>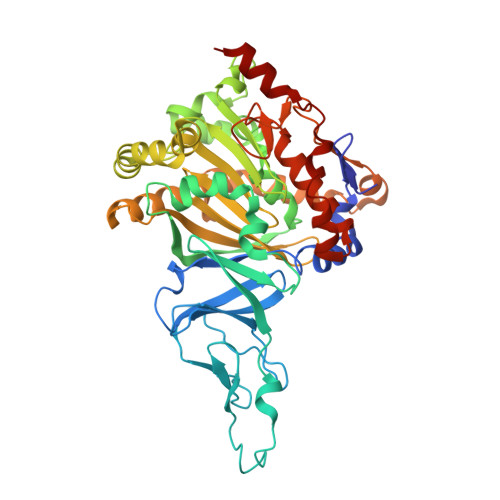 MSSDATLVDTVNASQSRQVFWDEDVYALEIERIFSRAWLMLGHESLVPKPGDFITTYMAEDKVILSHQSDGTFRAFINSCSHRGNQICHADSGNAKAFVCNYHGWVFGQDGSLVDVPLESRCYHNSLDKQKLAAKSVRVETYKGFIFGCHDPEAPSLEDYLGEFRYYLDTIWEGAGGGMELLGPPMKSLLQCNWKVPAENFIGDGYHVGWTHAAALSQIGGELAGLAGNRADIPFDDLGLQFTTRHGHGFGVIDNAAAGLHIKREGWTKFLEDTRGEVRRKFGPERERLYLGHWNCSIFPNCSFLYGTNTFKIWHPRGPHEIEVWTYTIVPRDADPATKSMIQREAIRTFGTAGTLESDDGENMSSATYINRGVITRNGRMNSTMGVGYEGPHPVYPGIVGISFIGETSYRGFYRFWKEMIDAPDWASVKANDDTWDSVFPNRNFWNEKLNAAE> QTGGSFYEPFNNYNTGLWQKADGYSNGNMFNCTWRANNVSMTSLGEMRLSLTSPSYNKFDCGENRSVQTYGYGLYEVNMKPAKNVGIVSSFFTYTGPTDGTPWDEIDIEFLGKDTTKVQFNYYTNGVGNHEKIVNLGFDAANSYHTYAFDWQPNSIKWYVDGQLKHTATTQIPQTPGKIMMNLWNGAGVDEWLGSYNG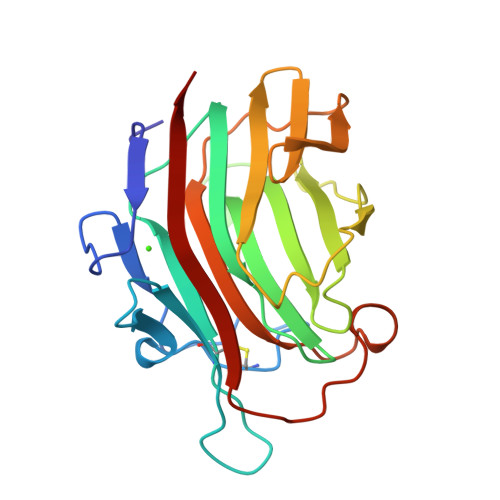VTPLYAHYNWVRYTKR N-[(1S,2R,3R,4R,5S)-2,3-dihydroxy-1-(hydroxymethyl)-6,8-dioxabicyclo[3.2.1]octan-4-yl]acetamide 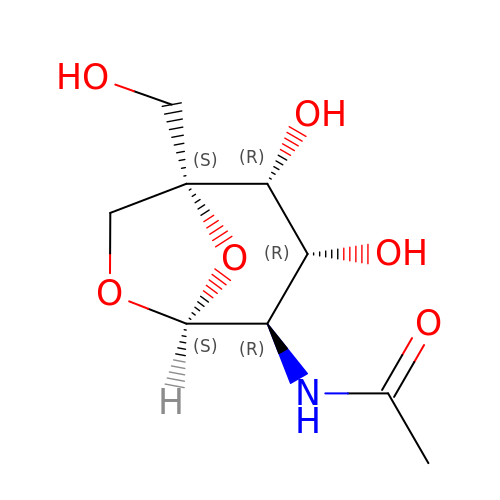| C9 H15 N O6 | HXIYAFJXGOVJDG-HXLXBVJFSA-N2-CHLORO-N-[[4-(3,5-DIMETHYLISOXAZOL-4-YL)PHENYL]METHYL]-1,4-DIMETHYL-1H-PYRAZOLE-4-SULFONAMIDE 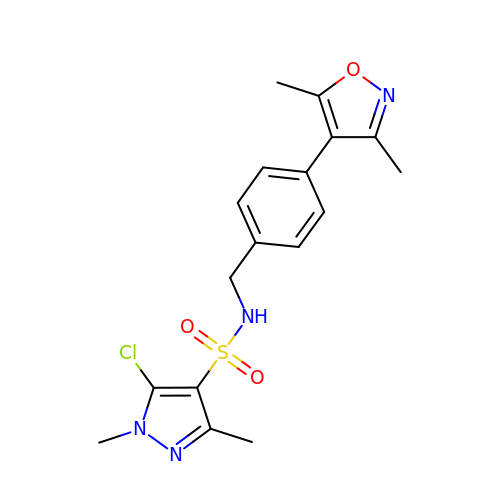| C17 H19 Cl N4 O3 S | XNTNHEPWXKNVBH-UHFFFAOYSA-N>MAFLADALSRVKPSATIAVSQKARELKAKGRDVIGLGAGEPDFDTPDNIKKAAIDAIDRGETKYTPVSGIPELREAIAKKFKRENNLDYTAAQTIVGTGGKQILFNAFMATLNPGDEVVIPAPYWVSYPEMVALCGGTPVFVPTRQENNFKLKAEDLDRAITPKTKWFVFNSPSNPSGAAYSHEELKALTDVLMKHPHVWVLTDDMYEHLTYGDFRFATPVEVEPGLYERTLTMNGVSKAYAMTGWRIGYAAGPLHLIKAMDMIQGQQTSGAASIAQWAAVEALNGPQDFIGRNKEIFQGRRDLVVSMLNQAKGISCPTPEGAFYVYPSCAGLIGKTAPSGKVIETDEDFVSELLETEGVAVVHGSAFGLGPNFRISYATSEALLEEACRRIQRFCAACR[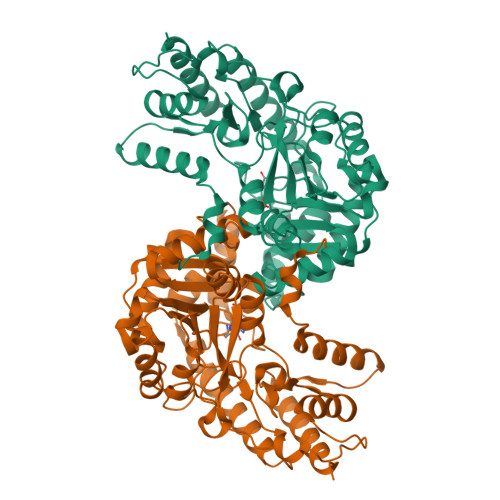6x]3,5,7,9,11-pentakis(oxidanylidene)dodecanal 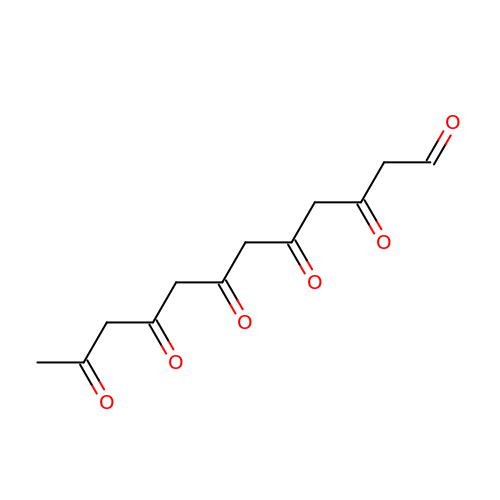| C12 H14 O6 | PTGARLKYUIIZKU-UHFFFAOYSA-N2-(4-HYDROXY-5-PHENYL-1H-PYRAZOL-3-YL)-1H-BENZOIMIDAZOLE-5-CARBOXAMIDINE 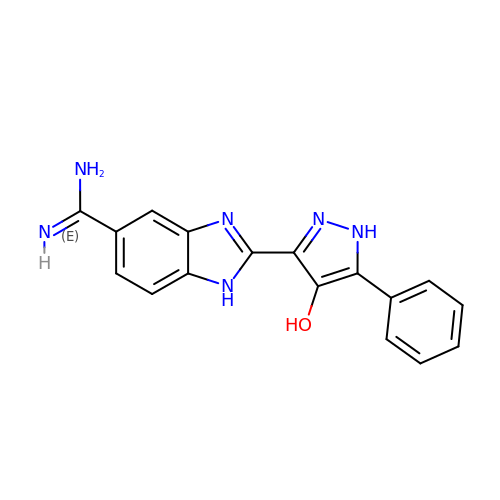| C17 H14 N6 O | CKSIVONWCYACAP-UHFFFAOYSA-N>[2x]GPAEPALREQQLQQELLALKQKQQIQRQILIAEFQRQHEQLSRQHEAQLHEHIKQQQEMLAMKHQQELLEHQRKLERHRQEQE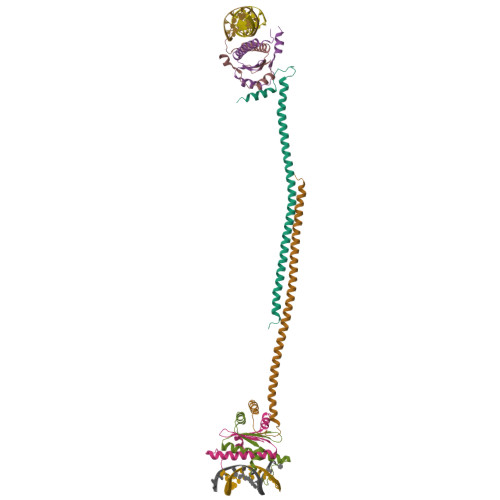LEKQHREQKLQQLKNKEKGKESAVASTEVKMKLQEFVLNKKKALAHRNLN;>GPMGRKKIQITRIMDERNRQVTFTKRKFGLMKKAYELSVLCDCEIALIIFNSSNKLFQYASTDMDKVLLKYTEYNEPHESRTNSDIVEALNKKEHRG[4x]>[2x]MGHHHHHHENLYFQGHMKNNKLGLRIGIVGGGISGVALALELCRYSHIQVQLFEAAPAFGEVGAGVSFGPNAVRAIVGLGLGEAYLQVADRTSEPWEDVWFEWRRGSDASYLGATIAPGVGQSSVHRADF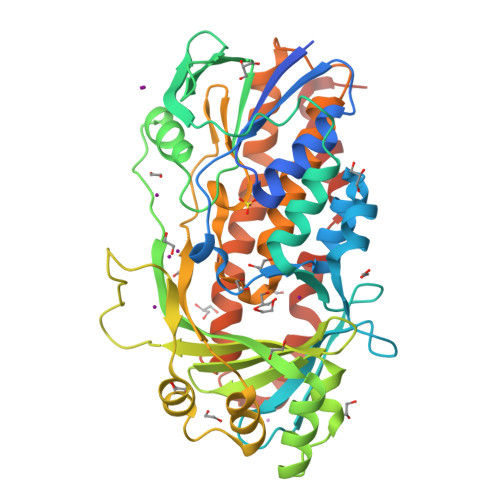IDALVTHLPEGIAQFGKRATQVEQQGGEVQVLFTDGTEYRCDLLIGADGIKSALRSHVLEGQGLAPQVPRFSGTCAYRGMVDSLHLREAYRAHGIDEHLVDVPQMYLGLDGHILTFPVRNGGIINVVAFISDRSEPKPTWPADAPWVREASQREMLDAFAGWGDAARALLECIPAPTLWALHDLAELPGYVHGRVVLIGDAAHAMLPHQGAGAGQGLEDAYFLARLLGDTQADAGNLAELLEAYDDLRRPRACRVQQTSWETGELYELRDPVVGANEQLLGENLATRFDWLWNHDLDTDLAEARARLGWEHGGGGALRQG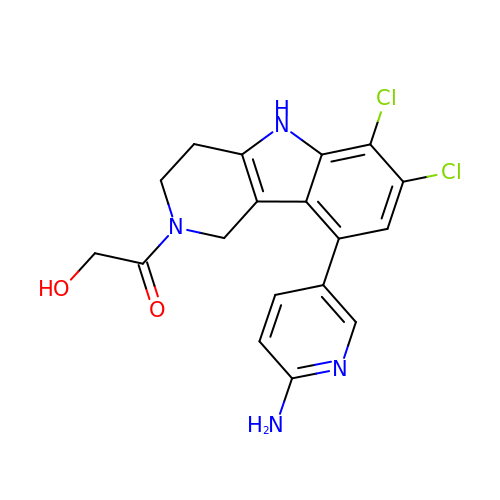1-[9-(6-aminopyridin-3-yl)-6,7-dichloro-1,3,4,5-tetrahydro-2H-pyrido[4,3-b]indol-2-yl]-2-hydroxyethan-1-one | C18 H16 Cl2 N4 O2 | VVUOUIPXYFIWLE-UHFFFAOYSA-N>KTISFNFNQFHQNEEQLKLQRDARISSNSVLELTKVVNGVPTWNSTGRALYAKPVQVWDSTTGNVASFETRFSFSIRQPFPRPHPADGLVFFIAPPNTQTGEGGGYFGIYNPLSPYPFVAVEFDTFRNTWDPQIPHIGIDVNSVISTKTVPFTLDNGGIANVVIKYDASTKILHVVLVFPSLGTIYTIADIVDLKQVLPESVNVGFSAATGD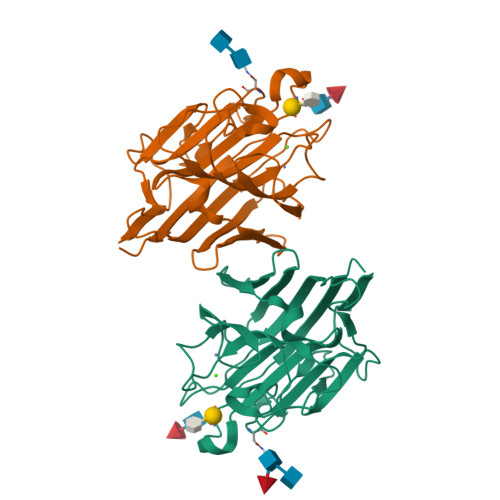PSGKQRNATETHDILSWSFSASLPGTNEF[4x]>[6x]GSHMSV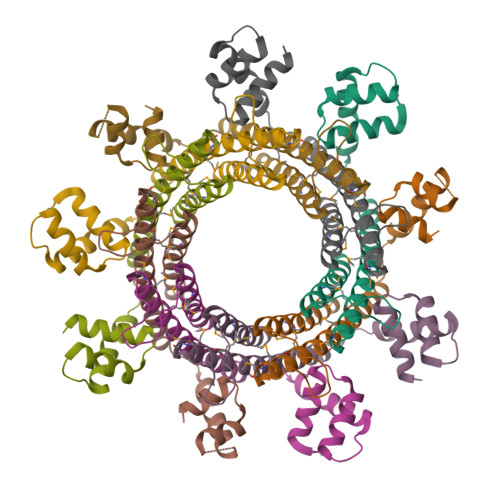SFRDRVLKLYLLGFDPSEIAQTLSLDVKRKVTEEEVLHVLAEARELLSALPSLEDIRAEVGQALERARIFQKDLLAIYQNMLRNYNAMMEGLTEHPDGTPVIGVRPADIAAMADRIMKIDQERITALLNSLKVLGHVGSTTAGALPSATELVSVEELVAEVVDEAPKT2,4-dibromo-6-{[(2-nitrobenzene-1-carbonyl)amino]methyl}phenyl 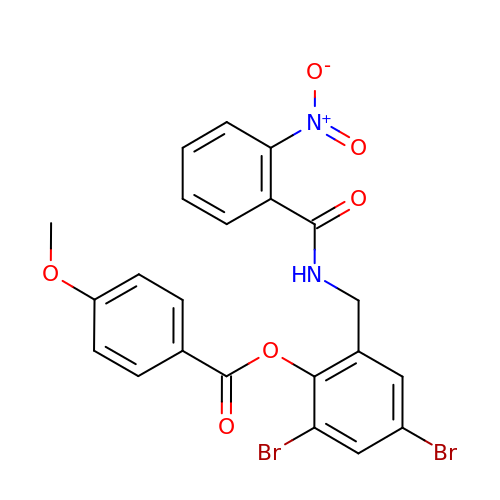4-methoxybenzoate | C22 H16 Br2 N2 O6 | ROLCPHUGRGJKFB-UHFFFAOYSA-N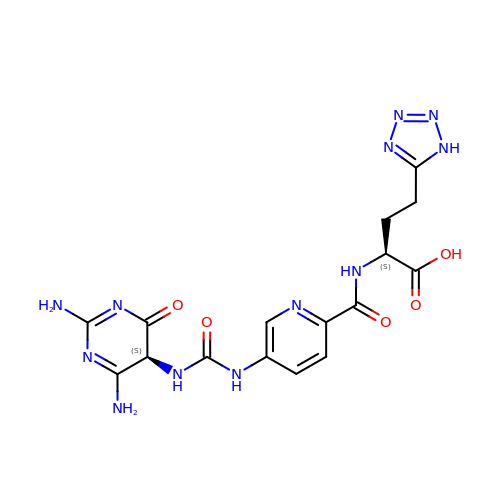(2~{S})-2-[[5-[[2,4-bis(azanyl)-6-oxidanylidene-5~{H}-pyrimidin-5-yl]carbamoylamino]pyridin-2-yl]carbonylamino]-4-(1~{H}-1,2,3,4-tetrazol-5-yl)butanoic acid | C16 H18 N12 O5 | AFYCZELCTVXAOG-WPRPVWTQSA-N> MPSFASLKSLVVLSLTSLSLAATVALDLHILNANLDPDGTGARSAVTAEGTTIAPLITGNIDDRFQINVIDQLTDANMRRATSIHWHGFFQAGTTEMDGPAFVNQCPIIPNESFVYDFVVPGQAGTYWYHSHLSTQYCDGLRGAFVVYDPNDPHLSLYDVDDASTVITIADWYHSLSTVLFPNPNKAPPAPDTTLINGLGRNSANPSAGQLAVVSVQSGKRYRFRIVSTSCFPNYAFS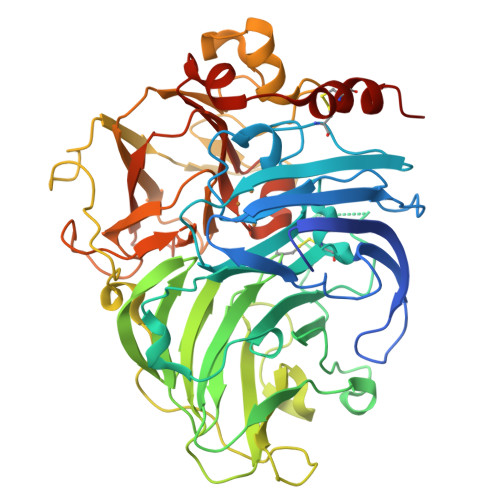IDGHRMTVIEVDGVSHQPLTVDSLTIFAGQRYSVVVEANQAVGNYWIRANPSNGRNGFTGGINSAIFRYQGAAVAEPTTSQNSGTALNEANLIPLINPGAPGNPVPGGADINLNLRIGRNATTADFTINGAPFIPPTVPVLLQILSGVTNPNDLLPGGAVISLPANQVIEISIPGGGNHPFHLHGHNFDVVRTPGSSVYNYVNPVRRDVVSIGGGGDNVTFRFVTDNPGPWFLHCHIDWHLEAGLAVVFAEDIPNIPIANAISPAWDDLCPKYNANNPDSGLA> MSEEEELATLSEEEIAMAVTAWEKGLESLPPLRPQQNPVLPVAGERNVLITSALPYVNNVPHLGNIIGCVLSADVFARYSRLRQWNTLYLCGTDEYGTATETKALEEGLTPQEICDKYHIIHADIYRWFNISFDIFGRTTTPQQTKITQDIFQQLLKRGFVLQDTVEQLRCEHCARFLADRFVEGVCPFCGYEEARGDQCDKCGKLINAVELKKPQCKVCRSCPVVQSSQHLFLDLPKLEKRLEEWLGRTLPGSDWTPNAQFITRSWLRDGLKPRCITRDLKWGTPVPLEGFEDKVFYVW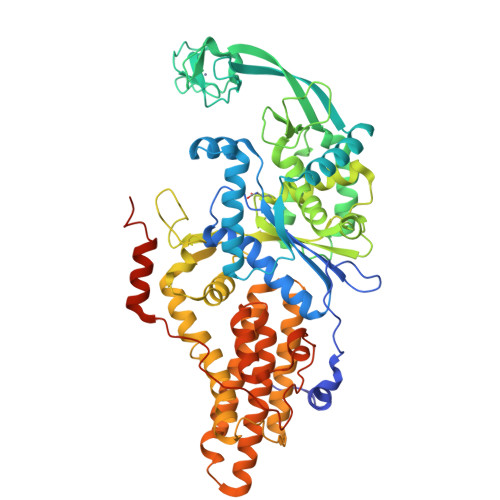FDATIGYLSITANYTDQWERWWKNPEQVDLYQFMAKDNVPFHSLVFPCSALGAEDNYTLVSHLIATEYLNYEDGKFSKSRGVGVFGDMAQDTGIPADIWRFYLLYIRPEGQDSAFSWTDLLLKNNSELLNNLGNFINRAGMFVSKFFGGYVPEMVLTPDDQRLLAHVTLELQHYHQLLEKVRIRDALRSILTISRHGNQYIQVNEPWKRIKGSEADRQRAGTVTGLAVNIAALLSVMLQPYMPTVSATIQAQLQLPPPACSILLTNFLCTLPAGHQIGTVSPLFQKLENDQIESLRQRFGGGQAKTSPKPAVVETVLEHHHHHH>GHQLPIWKQDEKSLTENDYYSFYKNTFKAYDDPLAYVHFNVEGQISFNSILYIPGSLPWELSKNMFDEESRGIRLYVKRVFINDKFSESIPRWLTFLRGIVDSENLPLNVGREILQKSKMLSIINKRIVLKSISMMKGLKETGGDKWTKFLNTFGKYLKIGVVEDKENQEEIASLVEFYSINSGDKKTDLDSYIENMKEDQKCIYYI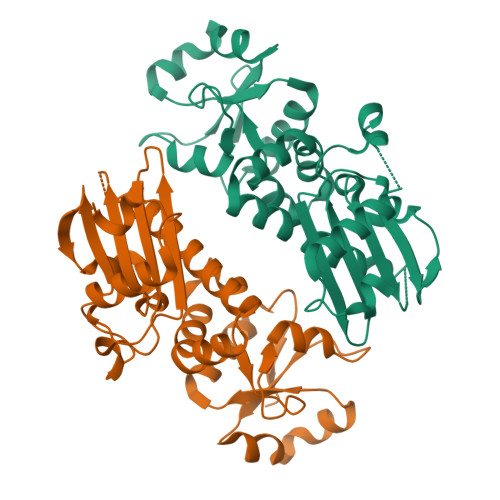SGENKKTAQNSPSLEKLKALNYDVLFSLEPIDEFCLSSLTVNKYKGYEVLDVNKAD[2x]>GPLGSMSDENKSTPIVKASDITDKLKEDILTISKDALDKYQLERDIAGTVKKQLDVKYGNTWHVIVGKNFGSYVTHEKGHFVYFYIGPLAFLVFKTA[3x];>[3x]ITY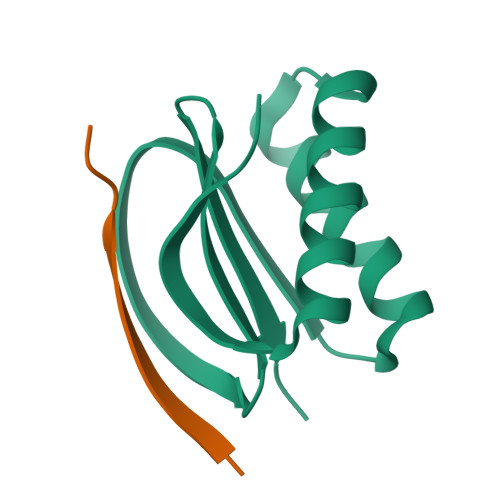DKGIQTDQ>[4x]SLHSPGKAFRAALTKENPLQIVGTINANHALLAQRAGYQAIYLSGGGVAAGSLGLPDLGISTLDDVLTDIRRITDVCSLPLLVDADIGFGSSAFNVARTVKSMIKAGAAGLHIEDQVGAKRSGHRPNKAIVSKEEMVDRIRAAVDAKTDPDFVIMARTDALAVEGLDAAIERAQAYVEAGAEMLFPEAITELAMYRQFADAVQVPILANITEFGAT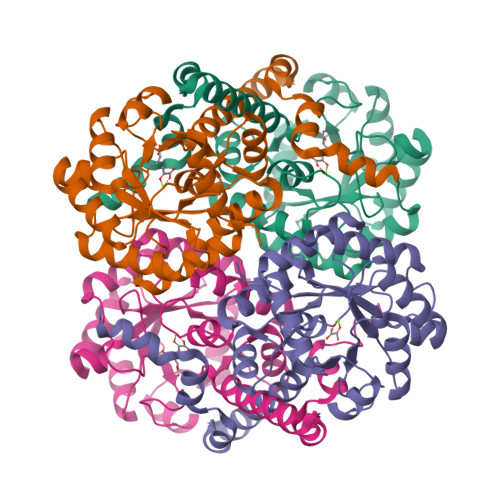PLFTTDELRSAHVAMALYPLSAFRAMNRAAEHVYNVLRQEGTQKSVIDTMQTRNELYESINYYQYEEKLDNLFARSQVK>[2x]GPGMAVKHLIVLKFKDEITEA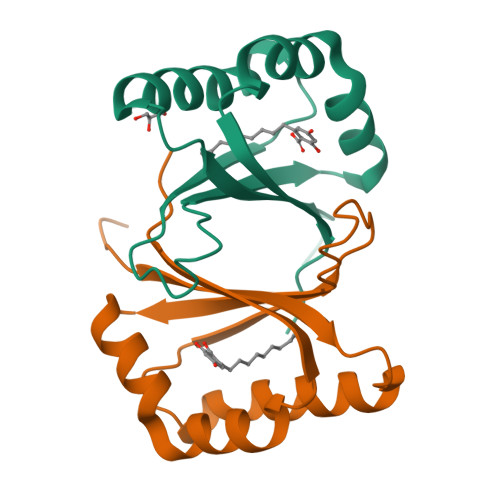QKEEFIKTYVNLVNIIPAMKDVYWGKDVTQKNKEEGYTHIVEVTFESVETIQDYIIHPAHVGFGDVYRSFWEKLLIFDYTPRK> SAKAAEGYEQIEVDVVAVWKEGYVYENRG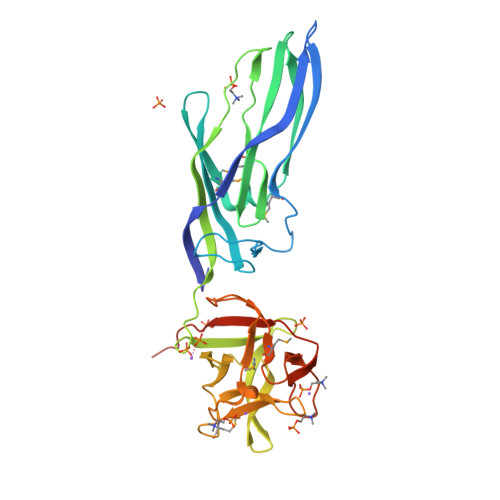STSVDQKITITKGMKNVNSETRTVTATHSIGSTISTGDAFEIGSVEVSYSHSHEESQVSMTETEVYESKVIEHTITIPPTSKFTRWQLNADVGGADIEYMYLIDEVTPIGGTQSIPQVITSRAKIIVGRQIILGKTEIRIKHAERKEYMTVVSRKSWPAATLGHSKLFKFVLYEDWGGFRIKTLNTMYSGYEYAYSSDQGGIYFDQGTDNPKQRWAINKSLPLRHGDVVTFMNKYFTRSGLCYDDGPATNVYCLDKREDKWILEVVGLVPRGSGHHHHHH> TTIVSVRRNGQVVVGGDGQVSLGNTVMKGNARKVRRLYNGKVLAGFAGGTADAFTLFELFERKLEMHQGHLLKSAVELAKDWRTDRALRKLEAMLIVADEKESLIITGIGDVVQPE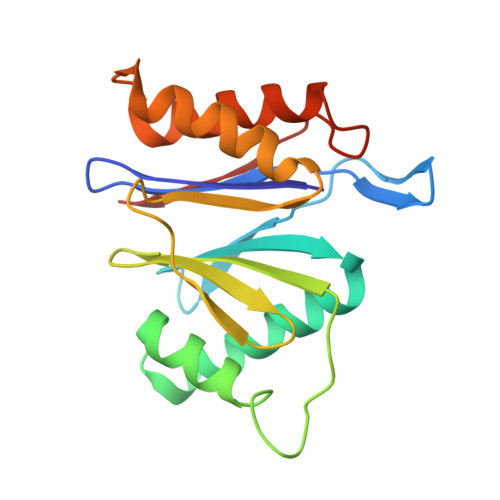EDQILAIGSGGNYALSAARALVENTELSAHEIVEKSLRIAGDICVFTNTNFTIEELPN> KFSKEQLRTFQMIHENFGRALSTYLSGRLRTFVDVEISIDQLTYEEFIRSVMIPSFIVIFTGDVFEGSAIFEMRLDLF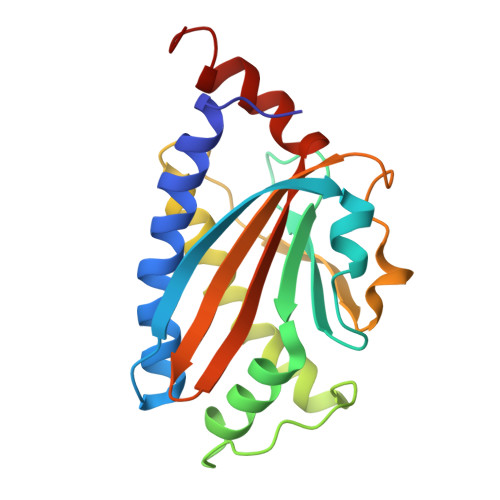YTMLDIIMGGPGENPPNRPPTEIETSIMRKEVTNMLTLLAQAWSDFQYFIPSIENVETNPQFVQIVPPNEIVLLVTASVSWGEFTSFINVCWPFSLLEPLLEKLSDRFWM>MAGIKVFGHPASIATRRVLIALHEKNLDFELVHVELKDGEHKKEPFLSRNPFGQVPAFEDGDLKLFESRAITQYIAHRYENQGTNLLQTDSKNISQYAIMAIGMQVEDHQFDPVASKLAFEQIFKSIYGLTTDEAVVAEEEAKLAKVLDVYEARLKEFKYLAGETFTLTDLHHIPAIQYLLGTPTKK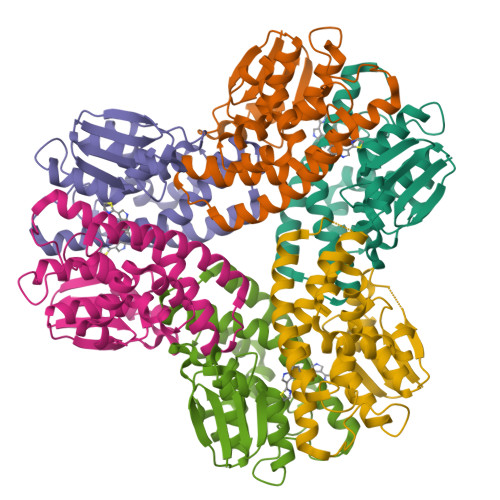LFTERPRVNEWVAEITKRPASEKVQ[24x]> MSTAKAPTLPASIFRAYDIRGVVGDTLTAETAYWIGRAIGSESLARGEPCVAVGRDGRLSGPELVKQLIQGLVDCGCQVSDVGMVPTP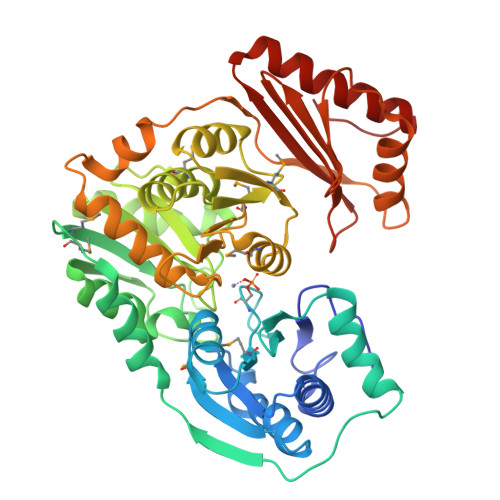VLYYAANVLEGKSGVMLTGSHNPPDYNGFKIVVAGETLANEQIQALRERIEKNDLASGVGSVEQVDILPRYFKQIRDDIAMAKPMKVVVDCGNGVAGVIAPQLIEALGCSVIPLYCEVDGNFPNHHPDPGKPENLKDLIAKVKAENADLGLAFDGDGDRVGVVTNTGTIIYPDRLLMLFAKDVVSRNPGADIIFDVKCTRRLIALISGYGGRPVMWKTGHSLIKKKMKETGALLAGEMSGHVFFKERWFGFDDGIYSAARLLEILSQDQRDSEHVFSAFPSDISTPEINITVTEDSKFAIIEALQRDAQWGEGNITTLDGVRVDYPKGWGLVRASNTTPVLVLRFEADTEEELERIKTVFRNQLKAVDSSLPVPF> MSNHTYRVIEIVGTSPDGVDAAIQNGL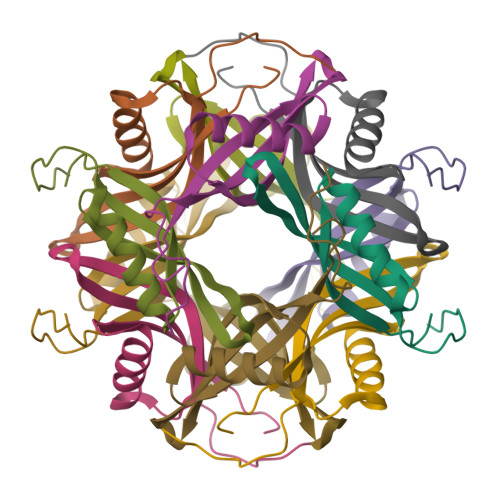ARAAQTMRALDWFEVQSIRGHLTDGTVAHFQVTMKVGFRLEDSGSGHHHHHH5-methyl-2-(2-propan-2-ylphenyl)-~{N}-(pyridin-2-ylmethyl)pyrrolo[3,2-d]pyrimidin-4-amine 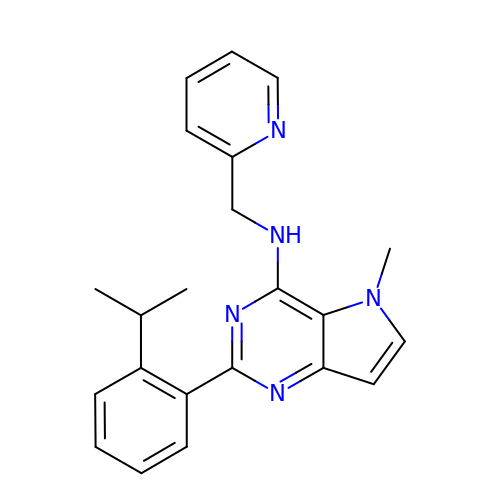| C22 H23 N5 | XIEZMAUGHWKZDR-UHFFFAOYSA-N>MSDAAPSLSNLFYDPTYNPGQSTINYTSIYGNGSTITFDELQGLVNSTVTQAIMFGVRCGAAALTLIVMWMTSRSRKTPIFIINQVSLFLIILHSALYFKYLLSNYSSVTYALTGFPQFISRGDVHVYGATNIIQVLLVASIETSLVFQIKVIFTGDNFKRIGLMLTSISFTLGIATVTMYFVSAVKGMIVTYNDVSATQDKYFNASTILLASSINFMSFVLVVKLILAIRSRRFLGLKQFDSFHILLIMSCQSLLVPSIIFILAYSLKPNQGTDVLTTVATLLAVLSLPLSSMWATAANNASKTNTITSDFTTSTDRFYPGTLSSFQTDSINNDAKSSLRSRLYDLYPRRKETTSDKHSERTFVSETADDIEKNQFYQLPTPTSSKNTR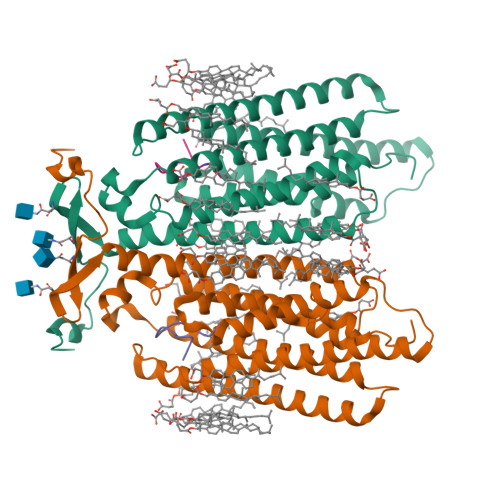IGPFADASYKEGEVEPVDMYTPDTAADEEARKFWTEDNNNL[2x];>[2x]HALQLKPGQPLY> MRDAVTTLIKNYDSTGRYLDRDAVDRLRSYFNS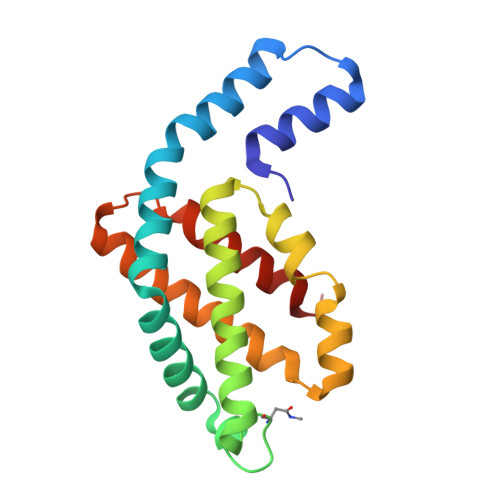GAARVKAAAVINANAAAIVKEAASALFTEQPELIQPGGNAYTTRRYATCLRDMDYYLRYASYAIVAGDVDVLNERVLEGLRETYNSLGVPIGPTVRGIQIMKEIVRDRVAAAGIEDTGIVEQPFDYMCRQLSEVNI Consistent with this, lrp6 mutant zebrafish lose asymmetry in the habenulae, and epistasis experiments support a role for Cachd1 in modulating Wnt pathway activity in the brain. These studies identify Cachd1 as a conserved Wnt receptor-interacting protein that regulates lateralized neuronal identity in the zebrafish brain. Biochemical and structural analyses demonstrated that Cachd1 can bind simultaneously to Lrp6 and Frizzled family Wnt co-receptors. Wnt ligands use FZDs and LRP5/6 receptors to initiate Wnt signaling. Our studies identify Cachd1 as a component of the Wnt pathway that bridges Fzd and Lrp6 Wnt receptors and plays an important role in the developing zebrafish brain.

Guided by our in vitro measurements, we attempted cocrystallization of CACHD1ECD with FZD5CRD and LRP6P3E3P4E4. Resultant crystals diffracted to 4.7Å resolution. There are three ternary complexes in an asymmetric unit (ASU). However, the CACHD1 structure reveals an addition to the C-terminal region of the ECD that does not show any homology to known structures in PDB by Dali search. This region interfaces with FZD5CRD and we therefore term it the FZD interaction (FZI) domain. The two α helices of the N-terminal dCache domain (C-1) interact with the LRP6P3 propeller. Thus, CACHD1 serves as a cross-linking component in the ternary complex, independently binding to FZD5CRD and LRP6P3E3P4E4. Structural superpositions show that the CACHD1 binding site on FZD5CRD overlaps with the “thumb” and palmitoleic acid (PAM) lipid binding site required for the receptor-ligand interaction with Wnt. Functional studies have indicated that LRP6P3E3P4E4 harbors the primary binding site for WNT3A and also for the C-terminal domain of DKK-1 (DKK-1C), an inhibitor that competes with Wnts for binding to LRP5/6 (23).

>[3x]MAREPEEEETVRPAAVVRRCPRCPGWPGAPRPPLWLLCLVACWILGAVADADFSILDEAQVLASQMRRLAAEELGVVTMQRIFNSLVYTEKISNGESEVQQLAKKIREKFNRYLDVVNRNKQVVEASYTAHLTSPLTAIQDCCTIPPSMMEFDGNFNTNVSRTVSCDRLSTTVNSRAFNPGRDLNSVLADNLKSNPGIKWQYFSSEEGIFTVFPAHKFRCKGSYEHRSRPIYVSTVRPQSKHIVVILDHGASVTDTQLQIAKDAAQVILSAIDEHDKISVLTVADAVRTCSLDQCYKTYLSPATSETKRKMSTFVSSVKPSDSPTQHAVGFHRAFQLIRSTSNSTRFQANTDMVIIYLSAGITSKDSSEEDKKATLRVINEENGFLNNSVMILTYALMNDGVTGLKELAFLRDLAEQNSGKYGIPDRTALPVIKGSMMVLNQLSNLETTVGRFYTNLPNRMIDEAVFSLPFSDEMGDGLIMTVSKPCYFGNLLLGIVGVDVNLAYILEDVTYYQDSLASYTFLIDDKGYTLMHPSLTRPYLLSEPPLHTDIIHYENIPKFELVRQNILSLPLGSQIITVPVNSSLSWHINKLRETGKEAYNVSYAWKMVQDTSFILCIVVIQPEIPVKQLKNLNTVPSSKLLYHRLDLLGQPSACLHFKQLATLESPTVMLSAGSFSSPYEHLSQPETKRMVEHYTAYLSDNTRLIANPGLKFSVRNEVMATSHVTDEWMTQMEMSSLNTYIVRRYIATPNGVLRIYPGSLMDKAFDPTRRQWYLHAVANPGLISLTGPYLDVGGAGYVVTISHTIHSSSTQLSSGHTVAVMGIDFTLRYFYKVLMDLLPVCNQDGGNKIRCFIMEDRGYLVAHPTLVDPKGHAPLEQQHITHKEPLVANDILNHPNFVKKNLCNSFSDRTVQRSYKFNTSLVGDLTNLVHGSHCSKYRLTRIPGTNAFVGIVNETCDSLAFCACSMVDRLCLNCHRMEQNECECPCECPLEVNECTGNLTNAENRNPSCEVHQEPVTYTAIDPGLQDALQQCVNSRCNQRMESGDCFGVLDCEWCVVDSDGKTHLDKSYCAPQKECFGGIVGAKSPYVDDMGATGLEVLFQ;>ETHASKAPVCQEITVPMCRGIGYNLTHMPNQFNHDTQDEAGLEVHQFWPLVEIHCSPDLRFFLCSMYTPICLPDYHKPLPPCRSVCERAKAGCSPLMRQYGFAWPERMSCDRLPVLGGDAEVLCMDYNRSEATGLEVLFQ[3x];>ETGVPEAFLLFSRRADIRRISLETNNNNVAIPLTGVKEASALDFDVTDNRIYWTDISLKTISRAFMNGSALEHVVEFGLDYPEGMAVDWLGKNLYWADTGTNRIEVSKLDGQHRQVLVWKDLDSPRALALDPAEGFMYWTEWGGKPKIDRAAMDGSERTTLVPNVGRANGLTIDYAKRRLYWTDLDTNLIESSNMLGLNREVIADDLPHPFGLTQYQDYIYWTDWSRRSIERANKTSGQNRTIIQGHLDYVMDILVFHSSRQSGWNECASSNGHCSHLCLAVPVGGFVCGCPAHYSLNADNRTCSAPTTFLLFSQKSAINRMVIDEQQSPDIILPIHSLRNVRAIDYDPLDKQLYWIDSRQNMIRKAQEDGSQGFTVVVSSVPSQNLEIQPYDLSIDIYSRYIYWTCEATNVINVTRLDGRSVGVVLKGEQDRPRAVVVNPEKGYMYFTNLQERSPKIERAALDGTEREVLFFSGLSKPIALALDSRLGKLFWADSDLRRIESSDLSGANRIVLEDSNILQPVGLTVFENWLYWIDKQQQMIEKIDMTGREGRTKVQARIAQLSDIHAVKELNLQEYRQHPCAQDNGGCSHICLVKGDGTTRCSCPMHLVLLQDELSCGGTKHHHHHH[3x]> P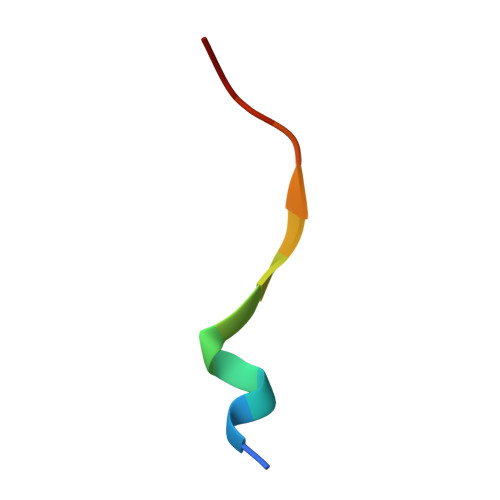ATGDFMNMSPVG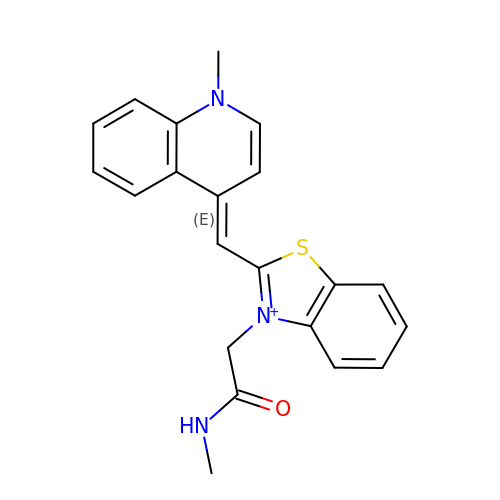~{N}-methyl-2-[2-[(~{E})-(1-methylquinolin-4-ylidene)methyl]-1,3-benzothiazol-3-yl]ethanamide | C21 H20 N3 O S | TZTFXKRTFIOKBN-UHFFFAOYSA-O(2R)-2-[(2-azanyl-4-oxidanylidene-3H-pteridin-7-yl)carbonylamino]-2-phenyl-ethanoic 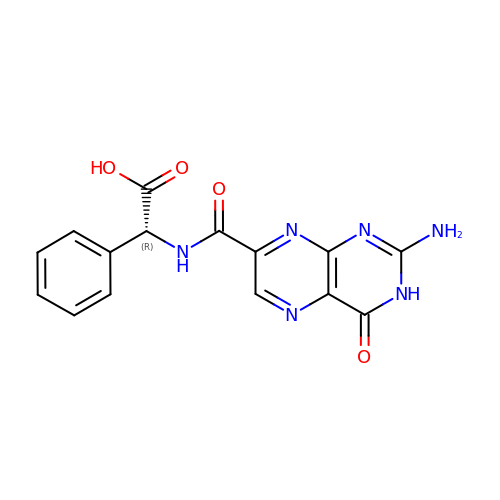acid | C15 H12 N6 O4 | CKTFFRDVMHUKQB-UHFFFAOYSA-N>AHAAIDTFTKYLDIDEDFATVLVEEGFSTLEELAYVPMKELLEIEGLDEPTVEALRERAKNALATIAQAQ[2x]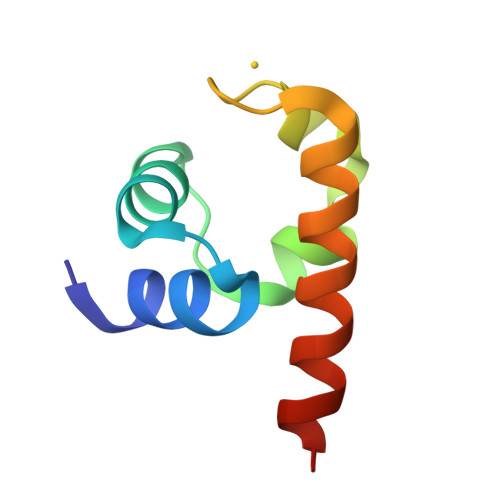;> NRPILSL> GTQNDRMP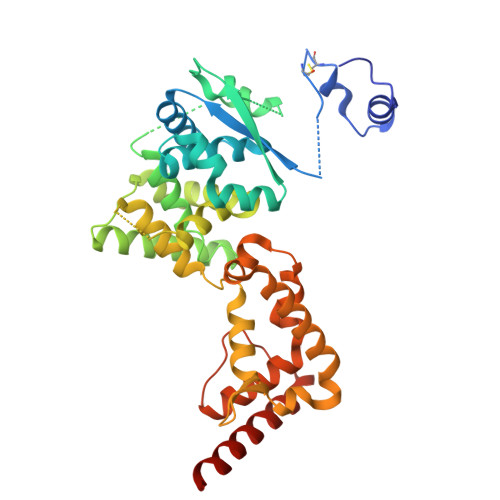GPELSGWISEQLMTGRIPVSDIFCDIENNPGLCYASQMQGIVRQRVIPVYQVNNLEEICQLIIQAFEAGVDFQESADSFLLMLCLHHAYQGDYKLFLESGAVKYLEGHGFRFEVKKRDGVKRLEELLPAVSSGKNIKRTLAAMPEEETTEANAGQFLSFASLFLPKLVVGEKACLEKVQRQIQVHAEQGLIQYPTAWQSVGHMMVIFRLMRTNFLIKFLLIHQGMHMVAGHDANDAVISNSVAQARFSGLLIVKTVLDHILQKTERGVRLHPLARTAKVKNEVNSFKAALSSLAKHGEYAPFARLLNLSGVNNLEHGLFPQLSAIALGVATAHGSTLAGVNVGEQYQQLREAATEAEKQLQQYAESRELDHLG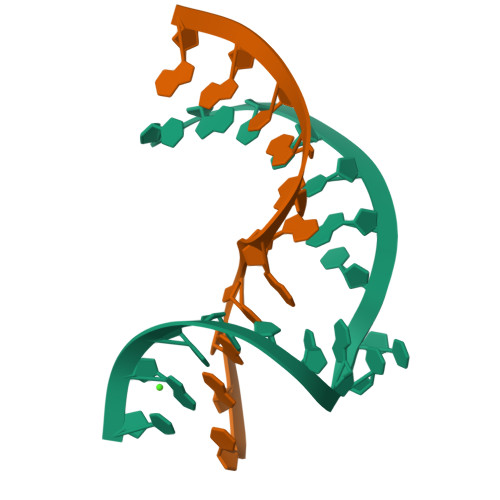>[2x]CGUCUACCCACCUCGC;>CGAGAGGACGG[2x]1-[3,4-bis(chloranyl)-5-methyl-indol-1-yl]ethanone 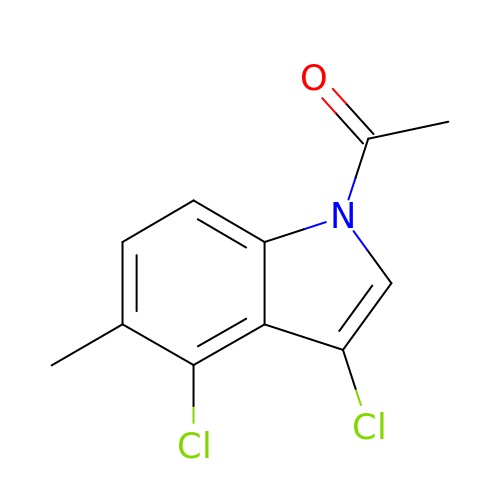| C11 H9 Cl2 N O | IETDZXPYBWJKDH-UHFFFAOYSA-N>MLNNWTEFVPAVKKAFGALGKQHPKMLAAYGALEEASAEGALDAKTRELISIAVAITTRCDGCIGVHTEAALKAGASEAEIAQTLATAISLNAGAAYVYSL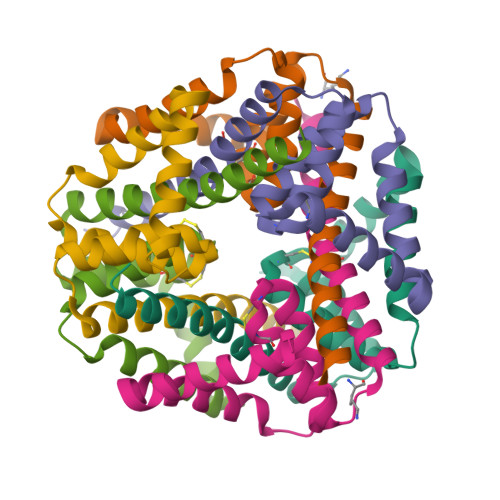RALEAYDQFKK[6x]> MKPKSGAVRRLEKNTMNFVLSDVADAEA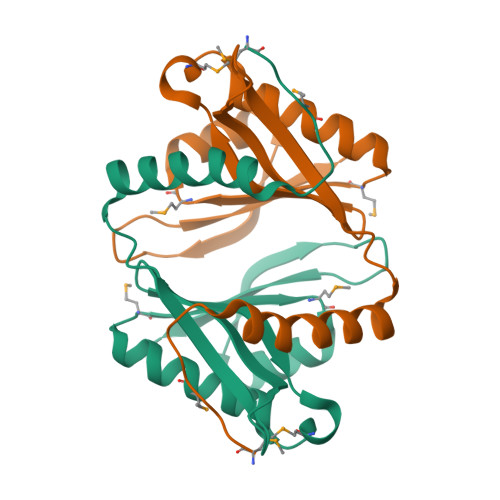EKAIRDPLVAYNLARFGESDKRDLNITIRNDDNSVTGGLVGHTARGWLYVQLLFVPEAMRGQGIAPKLLAMAEEEARKRGCMGAYIDTMNPDALRTYERYGFTKIGSLGPLSSGQSITWLEKRF5-methyl-1-(5-O-phosphono-beta-D-ribofuranosyl)-1,5-dihydro-1,4,5,6,8-pentaazaacenaphthylen-3-amine 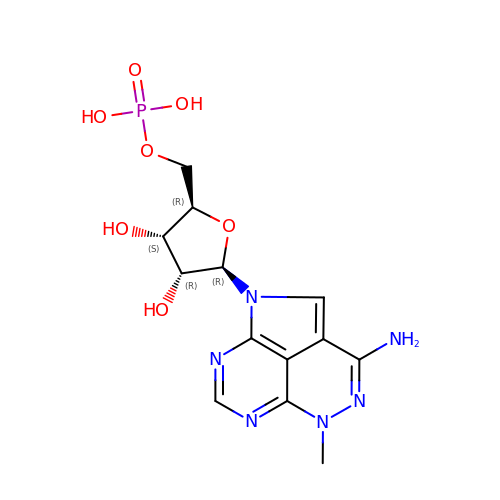| C13 H17 N6 O7 P | URLYINUFLXOMHP-HTVVRFAVSA-N> MAIYADNSYSIGNTPLVRLKHFGHNGNVVVKIEGRNPSYSVKCRIGANMVWQAEKDGTLTKGKEIVDATSGNTGI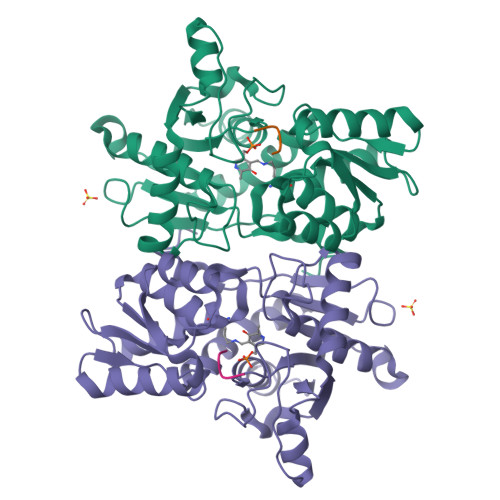ALAYVAAARGYKITLTMPETMSLERKRLLCGLGVNLVLTEGAKGMKGAIAKAEEIVASDPSRYVMLKQFENPANPQIHRETTGPEIWKDTDGKVDVVVAGVGTGGSITGISRAIKLDFGKQITSVAVEPVESPVISQTLAGEEVKPGPHKIQGIGAGFIPKNLDLSIIDRVETVDSDTALATARRLMAEEGILAGISSGAAVAAADRLAKLPEFADKLIVVILPSASERYLSTALFEGIEG;> GIDDGMNLNI2-[[7-[3-(aminomethyl)phenoxy]-1-methoxy-4-oxidanyl-isoquinolin-3-yl]carbonylamino]ethanoic acid | C20 H19 N3 O6 | 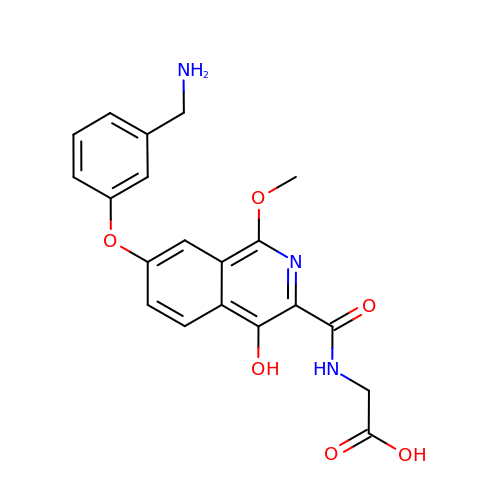MNBIZDSZQHYUGZ-UHFFFAOYSA-N> MKNKTELKKFYELLLAKLPKESVPILRTIFFSIRDGQAV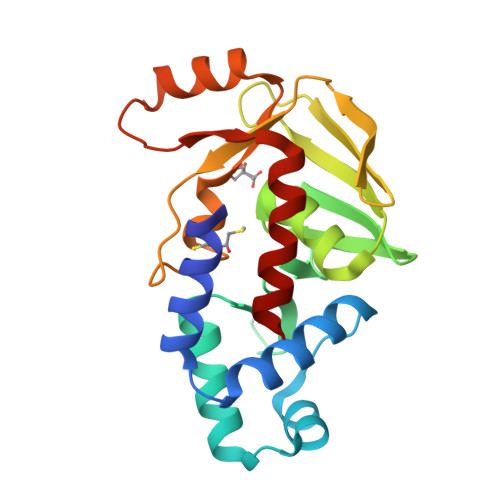TESSLINQTGINTKTVQSVVKILAQRQMIVREADQKIVGALGLSIIPTTNQIHLGGRTLFAWCAISTLELSTALVADVDIHSRCAYTGEPIEVTVRNGKLAKTTPDSTVIWTVPFDSEAPWAGGTCKQIHYFSSVEHANKWKEEHPKLQGEIMTLEQALSFGNELKKFLS> TDPIADMLTRIRNATRVYKESTDVPASRFKEEILRILAREGFIKGYERVDVDGKPYLRVYLKYGPRRQGPDPRPEQVIHHIRRISKPGRRVYVGVKEIPRVRRGLGIAILSTSKGVLTDREARKL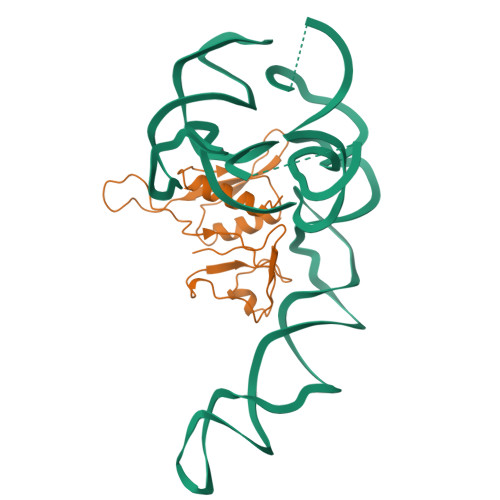GVGGELICEVW[4-[[6-(3,5-dimethyl-4-oxidanyl-phenyl)-[1,2,4]triazolo[1,5-a]pyridin-2-yl]amino]phenyl]-morpholin-4-yl-methanone | C25 H25 N5 O3 | 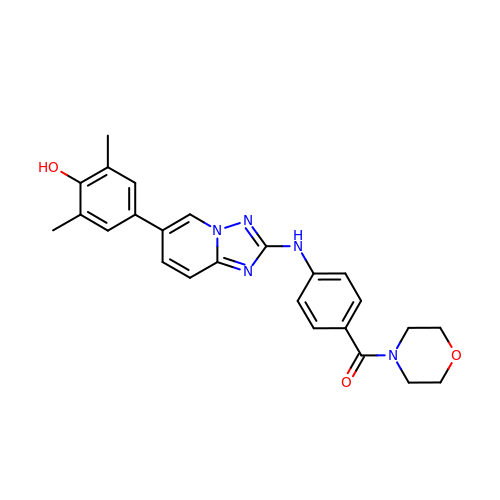SBPRNAZJEHULEN-UHFFFAOYSA-N>[4x]GPLGSMPSQMEHAMETMMFTFHKFAGDKGYLTKEDLRVLMEKEFPGFLENQKDPLAVDKIMKDLDQCRDGKVGFQSFFSLIAGLTIACNDYFVVHMKQENLYFQGDSTVHEILSKLS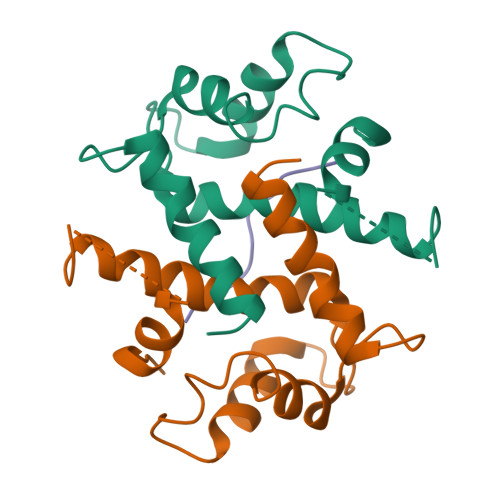LEGD;>GKVTFPKMKIPKFTFSGREL[2x]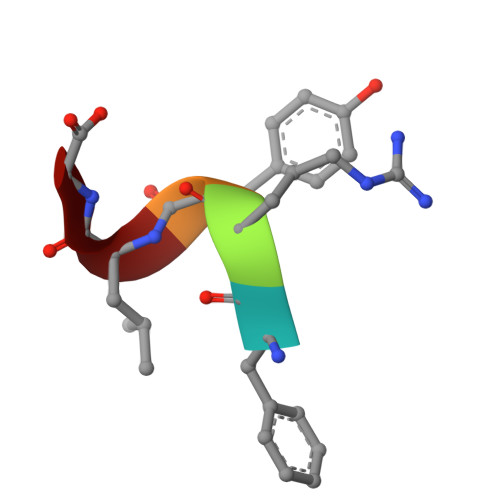> FRYLG> MNLTIKEEDFTNTFMKNEESFNTFRVTKVKRWNAKRLFKILFVTVFIVLAGGFSYYIFENFVFQKNRKINHIIKTSKYSTVGFNIENSYDRLMKTIKE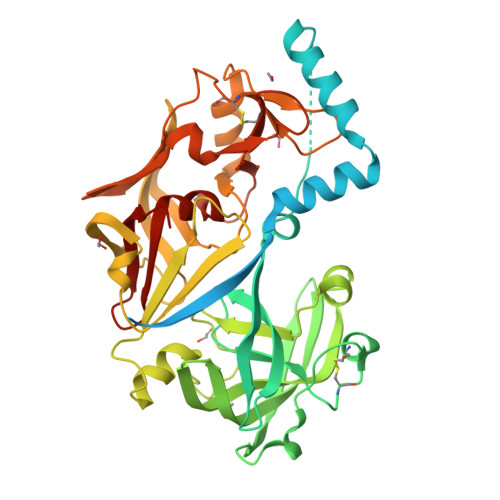HKLKNYIKESVKLFNKGLTKKSYLGSEFDNVELKDLANVLSFGEAKLGDNGQKFNFLFHTASSNVWVPSIKCTSESCESKNHYDSSKSKTYEKDDTPVKLTSKAGTISGIFSKDLVTIGKLSVPYKFIEMTEIVGFEPFYSESDVDGVFGLGWKDLSIGSIDPYIVELKTQNKIEQAVYSIYLPPENKNKGYLTIGGIEERFFDGPLNYEKLNHDLMWQVDLDVHFGNVSSKKANVILDSATSVITVPTEFFNQFVESASVFKVPFLSLYVTTCGNTKLPTLEYRSPNKVYTLEPKQYLEPLENIFSALCMLNIVPIDLEKNTFVLGDPFMRKYFTVYDYDNHTVGFALAKNL> QGAMEVLDINDNEPVFTQDVFVGSVEELSAAHTLVMKINATDADEPNTLNSKISYRIVSLEPAYPPVFYLNKDTGEIYTTSVTLDREE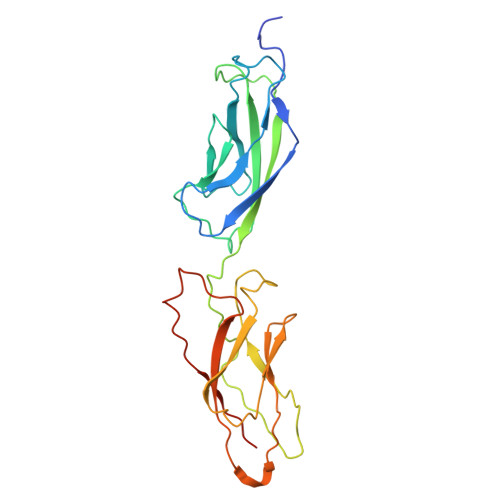HSSYTLTVEARDGNGEVTDKPVKQAQVQIRILDVNDNIPVVENKVLEGMVEENQVNVEVTRIKVFDADEIGSDNWLANFTFASGNEGGYFHIETDAQTNEGIVTLIKEVDYEEMKNLDFSVIVANKAAFHKSIRSKYKPTPIPIKVKVKNVKEGI>MRNEMHLQFSARSENESFARVTVAAFVAQLDPTMDELTEIKTVVSEAVTNAIIHGYNNDPNGIVSISVIIEDGVVHLTVRDEGVGIPDIEEARQPLFTTKPELERSGMGFTIMENFMDEVIVESEVNKGTTVYLKK[2x];>[2x]GSHMSLAIDLEVKQDVLIVRLSGELDHHTAEELREQVTDVLENRAIR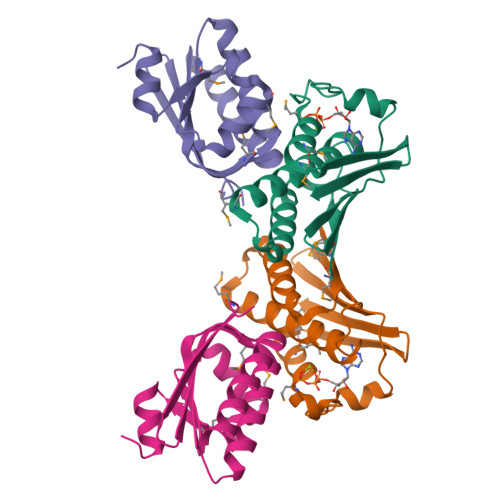HIVLNLGQLTFMDASGLGVILGRYKQIKNVGGQMVVCAVSPAVKRLFDMSGLFKIIRVEADEQFALQALGVA4-amino-4,6-dideoxy-alpha-D-glucopyranose | C6 H13 N O4 | 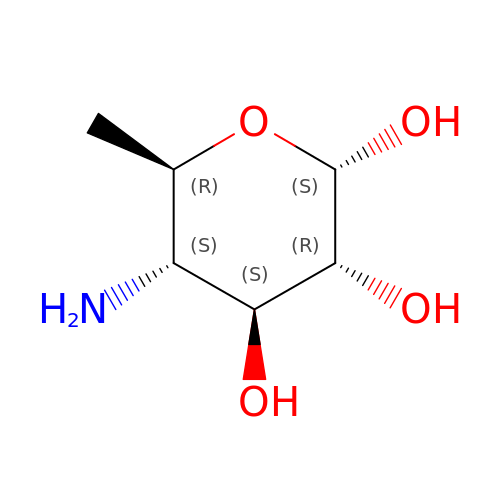RJKBJEZZABBYBA-DVKNGEFBSA-N5-[(4-{cis-4-[3-(trifluoromethyl)phenyl]cyclohexyl}piperazin-1-yl)methyl]pyridin-2(1H)-one | C23 H28 F3 N3 O | 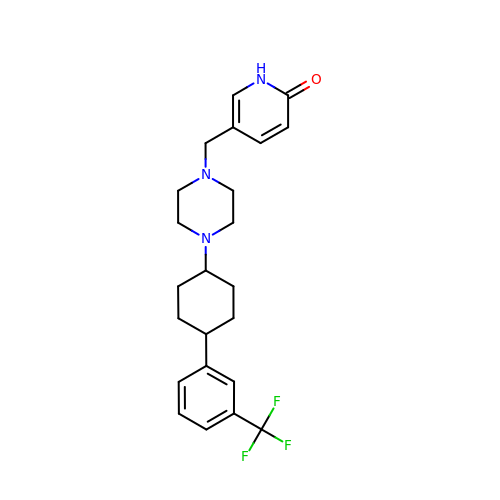DMSJDEOGYRYVRN-RVWIWJKTSA-N4-methyl-3-[(1-methyl-6-pyridin-3-yl-pyrazolo[3,4-d]pyrimidin-4-yl)amino]-~{N}-[3-(trifluoromethyl)phenyl]benzamide 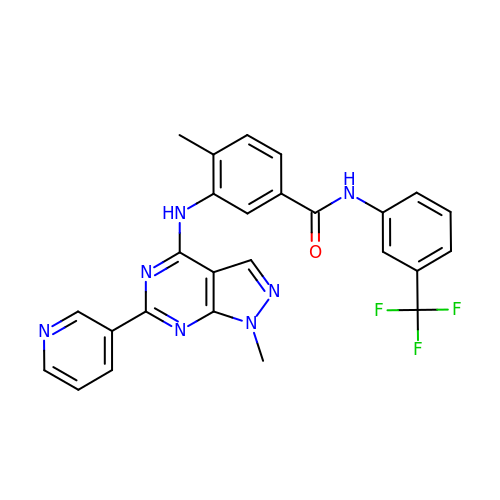| C26 H20 F3 N7 O | ZCCPLJOKGAACRT-UHFFFAOYSA-N Cytochrome P450 reductases (CPRs or CYPORs, EC 1.6.2.4) are diflavin oxidoreductases that supply electrons to type II cytochrome P450 monooxygenases (CYPs, EC 1.14.-.-). The structure is well conserved among the different kingdoms, possessing an N-terminal FMN-binding domain that is connected to a C-terminal FAD-binding domain via a linker region. The enzyme transfers electrons from NADPH in a typical order via flavin adenine dinucleotide (FAD) to flavin mononucleotide (FMN), which ultimately shuttles the electrons to the protein acceptors. Analysis of the CtCPR sequence revealed the presence of a single membrane-spanning region comprising the first 22 amino acids of the protein and in an attempt to produce more soluble CPR, a truncated, untagged version (Δ2–22) of the enzyme was expressed in E. coli.

The X-ray structures of CtCPR were solved with and without the cofactor, NADPH, at resolutions of 1.5 Å and 2.1 Å, respectively. Both structures were obtained in the closed conformation wherein the FMN-binding, flavodoxin-like domain interacts with the FAD and NADP- binding, ferredoxin-NADP+ reductase (FNR) like domain. In this conformation, the FMN and FAD moieties are in close proximity (~4.3 Å between the 7-methyl groups and ~3.6 Å between the 8-methyl groups), allowing direct electron transfer between the flavins. Despite the fact that CtCPR crystallized in the presence of excess NADPH, the open structure was not observed. No differences were detected between the two structures, with the exception of the presence of the 3′-phosphate-adenosine-5′-diphosphate part of NADPH, which, in contrast to the FMN and FAD cofactors, is bound through mostly side chain interactions. No density was observed for the nicotinamide mononucleotide moiety of the NAPDH, with the C-terminal Trp679 instead stacked on the re-side of the FAD. This residue is conserved among CPRs and has been implicated in the regulation of electron transfer. rCPR and hCPR have extended C-termini, with the equivalent tryptophan as the penultimate residue. As the tryptophan sterically prevents the binding of the nicotinamide part of NADPH, movement is required for hydride transfer to occur. The transition between the open and closed formations could limit hydride transfer from NADPH to FAD, as well as interflavin electron transfer, as the resting state of CPR appears to be the closed conformation during which NADPH binding occurs.

>[2x]MALDKLDLYVIITLVVAVAAYFAKNQFLDQPQDTGFLNTDSGSNSRDVLSTLKKNNKNTLLLFGSQTGTAEDYANKLSRELHSRFGLKTMVADFADYDWDNFGDITEDILVFFIVATYGEGEPTDNADEFHTWLTEEADTLSTLRYTVFGLGNSTYEFFNAIGRKFDRLLSEKGGDRFAEYAEGDDGTGTLDEDFMAWKDNVFDALKNDLNFEEKELKYEPNVKLTERDDLSAADSQVSLGEPNKKYINSEGIDLTKGPFDHTHPYLARITETRELFSSKERHCIHVEFDISESNLKYTTGDHLAIWPSNSDENIKQFAKCFGLEDKLDTVIELKALDSTYTIPFPTPITYGAVIRHHLEISGPVSRQFFLSIAGFAPDEETKKTFTRLGGDKQEFATKVTRRKFNIADALLYSSNNTPWSDVPFEFLIENIQHLTPRYYSISSSSLSEKQLINVTAVVEAEEEADGRPVTGVVTNLLKNIEIAQNKTGEKPLVHYDLSGPRGKFNKFKLPVHVRRSNFKLPKNSTTPVILIGPGTGVAPLRGFVRERVQQVKNGVNVGKTLLFYGCRNSNEDFLYKQEWAEYASVLGENFEMFNAFSRQDPSKKVYVQDKILENSQLVHELLTEGAIIYVCGDASRMARDVQTTISKIVAKSREISEDKAAELVKSWKVQNRYQEDVW> HHHHHHEEKNYHQPAILNSSALRQIAEGTSISEMWQNDLQPLLIERYPG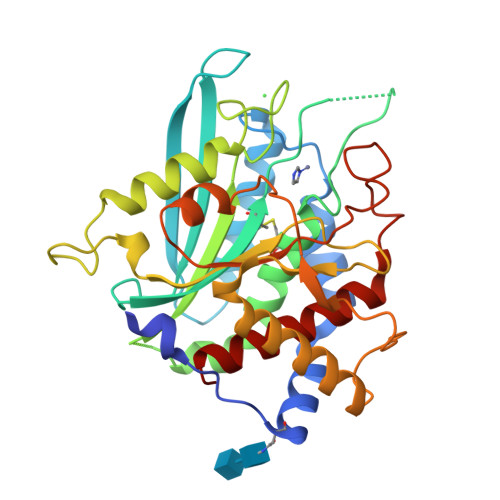SPGSYAARQHIMQRIQRLQADWVLEIDTFLSQTPYGYRSFSNIISTLNPTAKRHLVLACHYDSKYFSHWNNRVFVGATDSAVPCAMMLELARALDKKLLSLKTVSDSKPDLSLQLIFFDGEEAFLHWSPQDSLYGSRHLAAKMASTPHPPGARGTSQLHGMDLLVLLDLIGAPNPTFPNFFPNSARWFERLQAIEHELHELGLLKDHSLEGRYFQNYSYGGVIQDDHIPFLRRGVPVLHLIPSPFPEVWHTMDDNEENLDESTIDNLNKILQVFVLEYLHL Sigma (σ) factors are bacterial protein modules that plug into RNA polymerase (RNAP) to recruit the enzyme to specific programs of gene transcription via recognition of promoter DNA and the subsequent initiation of transcription. The vast majority of σ factors are members of the σ70 protein superfamily, which is subdivided into four classes based upon their extent of conservation and the presence/absence of the conserved σ domains (σ1.1, σ2, σ3, and σ4 connected by flexible loop regions) that mediate interactions with RNAP and/or promoter DNA. In B. subtilis there are four sigma factors known to control sporulation—the process in which the bacteria become long-lived dormant spores to survive stress conditions. The sigma factor “puppeteers” involved in this process are SigF in the forespore and SigE in the mother cell at the early phases; then, these are replaced by SigG and SigK, respectively, as sporulation progresses.

Here we present an experimentally solved X-ray crystal structure of SigE residues 17–133 and review all of the available experimentally-solved and AlphaFold-predicted B. subtilis sigma factor structures. Initially we produced almost full-length B. subtilis SigE (residues 17–239, only missing the initial prosequence that maintains SigE in an inactive state before processing), but we found that it degraded to a smaller domain that remained stable over time, as observed by SDS-PAGE and 2D NMR. Smaller constructs were designed based on predicted domain boundaries, and SigE17–133 was the variant that successfully yielded diffracting crystals. The first 27 residues of SigE are a pro-sequence that keeps the protein in the inactive state and ensures its localization to the mother cell. These residues get cleaved during sporulation by SpoIIGA to activate the protein. The constructs used in this study lack the first 17 residues as this maintains activity in vivo without requiring processing by SpoIIGA. Crystals grew over a period of 4–6 months and the protein likely lost some N-terminal amino acids during this process. It is also possible that these residues were too flexible to give rise to discernible electron density. The structure is a classic four helix-turn-helix core found in all sigma factor σ2 domains and covers regions σ2.1 (55–78), σ2.2 (79–97), and σ2.3 (98–117) of SigE, which includes the binding sites for both CsfB and the −10 promoter DNA sequence for transcriptional activation. The solved structure aligns very well (RMSD: 0.51 Å) with the AlphaFold prediction for SigE, with Alphafold providing a slight helix overprediction in the loop between two helices.

>[6x]PNGDQAARAILIERNLRLVVYIARKFENTGINIEDLISIGTIGLIKAVNTFNPEKKIKLATYASRCIENEILMYLRRNNKIR> MSRQMWLDTSALLEAISEYVVRCNGDTFSGLTTGDFNALSNMFTQLSVSSAGYVSDPRVPLQTMSNMFVSFITSTDRCGYMLRKTWFNSDTKPTVSDDFITTYIRPRLQVPMSDTVRQLNNLSLQPSAKPKLYERQNAIMKGLDIPYSEPIEPCKLFRSVAGQTGNIPMMGILATPPAAQQQPFFVAERRRILFGIRSNAAIPAGAYQFVVPAWASVLSVTGAYVYFTNSFFGTIIAGVTATATAADAATTFTVPTDANNLPVQTDSRLSFSLGGGNINLELGVAKTGFCVAIEGEFTILANRSQAYYTLNSITQ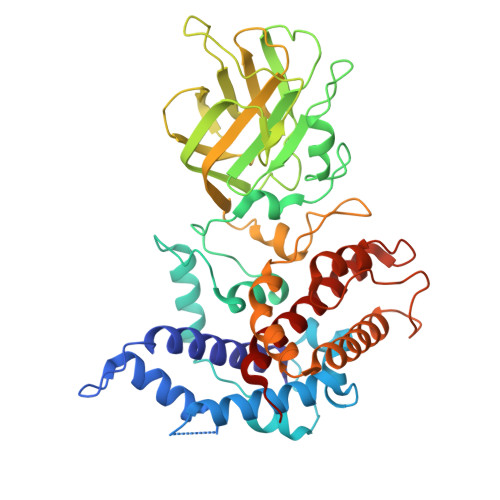TPTSIDDFDVSDFLTTFLSQLRACGQYEIFSDAMDQLTNSLITNYMDPPAIPAGLAFTSPWFRFSERARTILALQNVDLNIRKLIVRHLWVITSLIAVFGRYYRPN> GAASRLRSPSVLEVREKG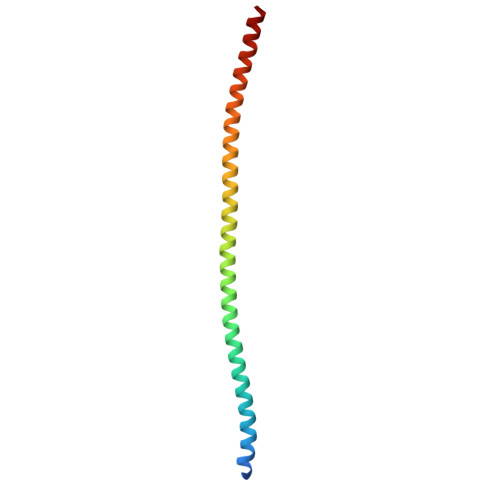YERLKEELAKAQRELKLKDEECERLSKVRDQLGQELEELTASLFEEAHKMVREANIKQATAEKQLKEAQGKIDVLQAEVAALKTLVLS>[2x]GSHHHHHHSQDPM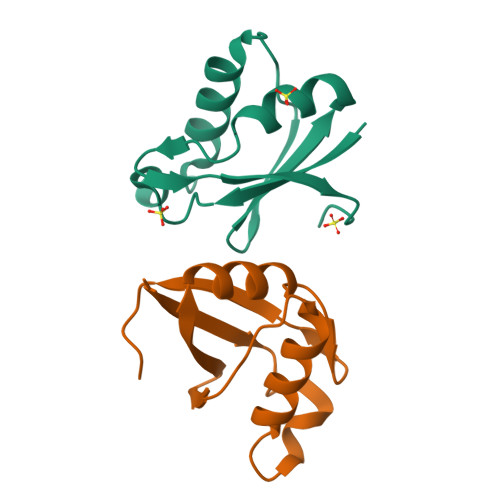KTQPNKTVIKILGLKNSKAASNPDGGLRSLLDFLERKSKEKITLGRGIIDGDYVWLKVNKDDAQHLLRLNGFTYAGATLTIEETNEPMPALSSQSKLSQAAQETKQKL>MAVDPILSSPLGPAASEKDAKALQFIEEMTRNADSVQERVLAEILSRNGETEYLKRFKLEGSTVRETFKSKIPVIKYEDLQPEIQRIANGDRSAILSAHPISEFLTSSGTSAGERKLMPTIQEELDRRQMLYSLLMPVMNLYVPGLDKGKGLYFLFVKSETRTPGGLLARPVLTSYYKSEHFKTRPYDPYNVYTSPNEAILCADSFQSMYTQMLCGIYERKQVLRLGAVFASGLLRAIRFLQLNWHQLTHDIRTGTLSPKITDPSVRNCVAGVLKPDPELADLVAGECSKDNWEGIITRIWPNTKYLDVIVTGAMAQYIPTLDYYSGGLPLACTMYASSECYFGLNLNPMSKPSEVSYTIMPNMAYFEFLPHEHSSIPLSRDSPPRLVDLAHVEVGKEYELVITTYAGLYRYRVGDILRVTGFHNSAPQFHFVRRKNVLLSIDSDKTDEAELQKAVDNASKLLREVNTSVVEYTSFADTKTIPGHYVIYWELLVKDSANSPSDELLGQCCLAMEESLNSVYRQGRVADNSIGPLEIRVVKSGTFEELMDYAISRGASINQYKVPRCVNFTPIMELLDSRVVSSHFSPALPHWTPARRR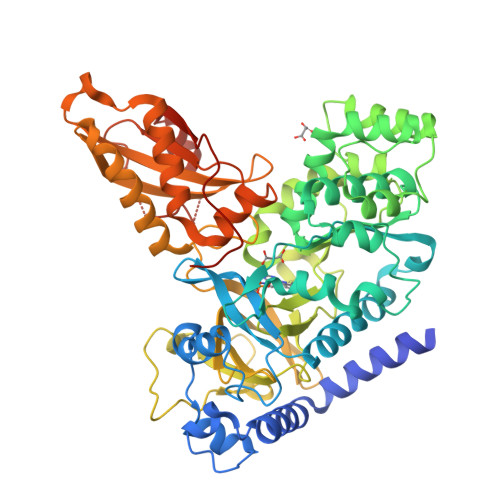AAALEHHHHHH[2x]Botulinum neurotoxin A1 (BoNT/A1) belongs to the most potent toxins and is used as a major therapeutic agent. BoNTs and BoNT-like proteins share a common domain organization and are produced as precursors that are cleaved into a 50 kDa light chain (LC) and a 100 kDa heavy chain (HC) that with the exception of BoNT/Wo remain connected by a disulfide bond. The LC is a zinc metalloprotease that specifically cleaves soluble N-ethylmaleimide-sensitive-factor attachment receptor (SNARE) proteins. While the physiological functions of SV2 proteins remains to be determined, their best-established role is to act as receptors for several BoNTs (BoNT/A, /D, /E, and /F).

The resulting refined 3D reconstructions of SV2B-HCA1 and SV2B-BoNT/A1 complexes were obtained at 3.7 Å and 4 Å resolution, respectively. Our description of the SV2B structure is therefore based on the cryo-EM reconstruction of the SV2B-HCA1 complex, which features a very well resolved density for the complete TM region of SV2B. A substantial portion of the receptor spanning amino-acid residues D87 to Q345 and R362 to E679 could be resolved by cryo-EM, confirming that the N-terminus of the protein is unstructured. The overall SV2 fold consists of three parts: the LD, the transmembrane domain (TM) and the intracellular structure comprising four helices. The most prominent feature of SV2B is the unique and characteristic LD located between TM7 and TM8. The conserved cysteine in the LD region, C526, forms a disulfide bridge with C141 in the luminal loop 1 (LL1). In contrast, the experimentally determined cryo-EM structure is closed, with the entrance to the putative solute translocation pathway sealed by LL1. Superimposition of the SV2B-HCA1 and gSV2C-LD-HCA1 structures revealed similar protein-carbohydrate interactions. Both structures share a complex-type N-glycan that is linked to Asn-516 with two N-acetylglucosamines (NAG), two mannoses (BMA) and a fucose (FUC). The most prominent feature of the direct interaction of the glycan at N516 and HCA1 is a π-CH stacking interaction between F953 and the sugar ring of the first NAG. Among these, the most prominent is a network of salt bridges and hydrogen bonds involving E521 of SV2B and Y1122, K1137, and R1156 of BoNT/A1.

> MDDYKYQDNYGGYAPSDGYYRGNESNPEEDAQSDVTEGHDEEDEIYEGEYQGIPHPDDVKAKQAKMAPSRMDSLRGQTDLMAERLEDEEQLAHQYETIMDECGHGRFQWILFFVLGLALMADGVEVFVVSFALPSAEKDMCLSSSKKGMLGMIVYLGMMAGAFILGGLADKLGRKRVLSMSLAVNASFASLSSFVQGYGAFLFCRLISGIGIGGALPIVFAYFSEFLSREKRGEHLSWLGIFWMTGGLYASAMAWSIIPHYGWGFSMGTNYHFHSWRVFVIVCALPCTVSMVALKFMPESPRFLLEMGKHDEAWMILKQVHDTNMRAKGTPEKVFTVSNIKTPKQMDEFIEIQSSTGTWYQRWLVRFKTIFKQVWDNALYCVMGPYRMNTLILAVVWFAMAFSYYGLTVWFPDMIRYFQDEEYKSKMKVFFGEHVYGATINFTMENQIHQHGKLVNDKFTRMYFKHVLFEDTFFDECYFEDVTSTDTYFKNCTIESTIFYNTDLYEHKFINCRFINSTFLEQKEGCHMDLEQDNDFLIYLVSFLGSLSVLPGNIISALLMDRIGRLKMIGGSMLISAVCCFFLFFGNSESAMIGWQCLFCGTSIAAWNALDVITVELYPTNQRATAFGILNGLCKFGAILGNTIFASFVGITKVVPILLAAASLVGGGLIALRLPETREQVLM;> MKKHHHHHHGSLVPRGSKNIINTSILNLRYESNHLIDLSRYASKINIGSKVNFDPIDKNQIQLFNLESSKIEVILKNAIVYNSMYENFSTSFWIRIPKYFNSISLNNEYTIINCMENNSGWKVSLNYGEIIWTLQDTQEIKQRVVFKYSQMINISDYINRWIFVTITNNRLNNSKIYINGRLIDQKPISNLGNIHASNNIMFKLDGCRDTHRYIWIKYFNLFDKELNEKEIKDLYDNQSNSGILKDFWGDYLQYDKPYYMLNLYDPNKYVDVNNVGIRGYMYLKGPRGSVMTTNIYLNSSLYRGTKFIIKKYASGNKDNIVRNNDRVYINVVVKNKEYRLATNASQAGVEKILSALEIPDVGNLSQVVVMKSKNDQGITNKCKMNLQDNNGNDIGFIGFHQFNNIAKLVASNWYNRQIERSSRTLGCSWEFIPVDDGWGERPL>[2x]MHHHHHHGSLVPRGSMDYKDDDDKENLYFQGSKKIFKPEELRQALMPTLEALYRQDPESLPFRQPVDPQLLGIPDYFDIVKNPMDLSTIKRKLDT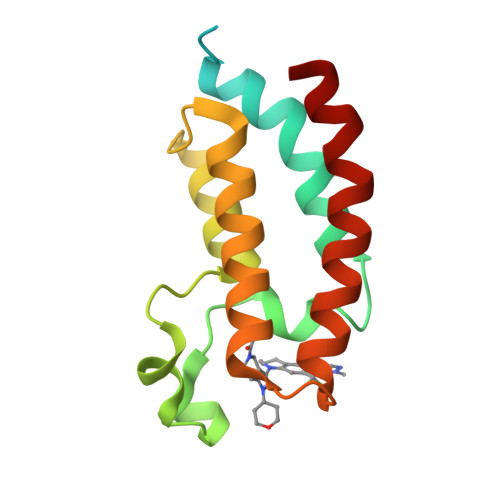GQYQEPWQYVDDVWLMFNNAWLYNRKTSRVYKFCSKLAEVFEQEIDPVMQSLG~{N}-[(2~{S})-1-(3-azanylpropylamino)-4-methyl-1-oxidanylidene-pentan-2-yl]-(phenylmethoxycarbonylaminomethyl)phosphonamidic 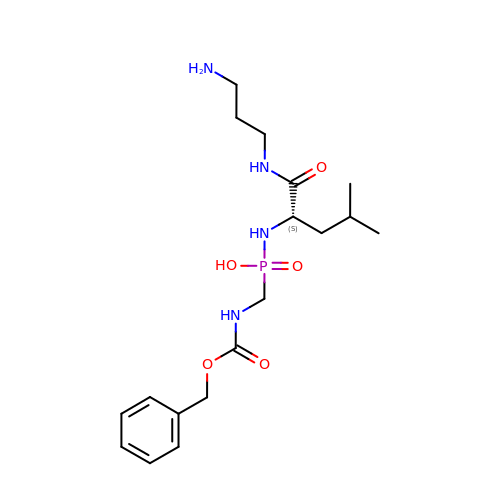acid | C18 H31 N4 O5 P | YXKYWNUEXNHFHI-INIZCTEOSA-N>[2x]MSFTPANRAYPYTRLRRNRRDDFSRRLVRENVLTVDDLILPVFVLDGVNQRESIPSMPGVERLSIDQLLIEAEEWVALGIPALALFPVTPVEKKSLDAAEAYNPEGIAQRATRALRERFPELGIITDVCLCPFTTHGQCGILD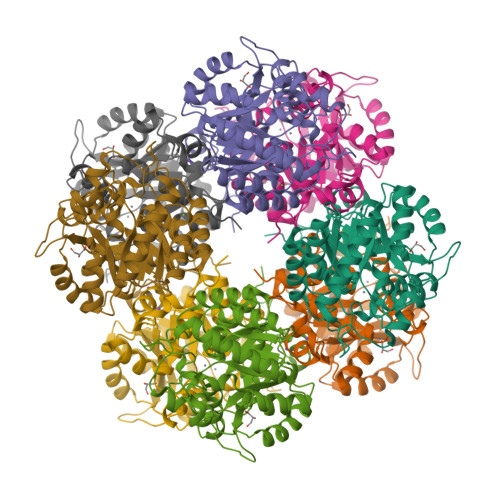DDGYVLNDVSIDVLVRQALSHAEAGAQVVAPSDMMDGRIGAIREALESAGHTNVRVMAYSAKYASAYYGPFRDAVGSASNLGKGNKATYQMDPANSDEALHEVAADLAEGADMVMVKPGMPYLDIVRRVKDEFRAPTFVYQVSGEYAMHMGAIQNGWLAESVILESLTAFKRAGADGILTYFAKQAAEQLRRGR> GAMEMSSANTNTSSAPDAPPRAVMKVAV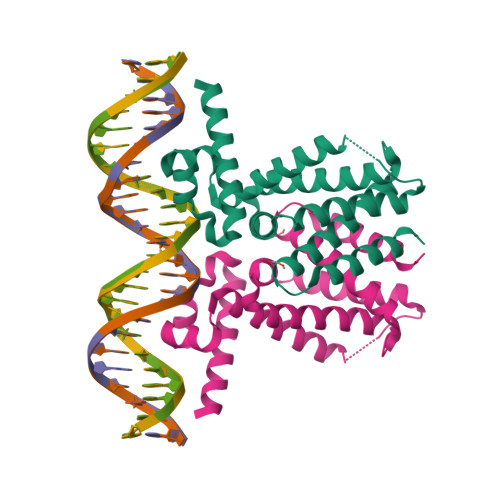LAESELGSEAQRERRKRILDATMAIASKGGYEAVQMRAVADRADVAVGTLYRYFPSKVHLLVSALGREFSRIDAKTDRSAVAGATPFQRLNFMVGKLNRAMQRNPLLTEAMTRAYVFADASAASEVDQVEKLIDSMFARAMANGEPTEDQYHIARVISDVWLSNLLAWLTRRASATDVSKRLDLAVRLLIGDQDSA> MPAVLGFEGSANKIGVGVVRDGKVLANPRRTYVTPPGTGFLPGDTARHHRAVILDLLQEALTESGLTSQDIDCIAYTKGPGMGAPLVSVAVVARTVAQLWNKPLVGVNHCIGHIEMGRLITGATSPTVLYVSGGNTQVIAYSEHRYRIFGETIDIAVGNCLDRFAR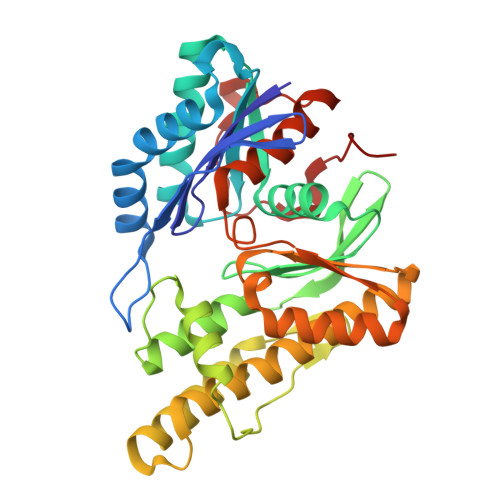VLKISNDPSPGYNIEQMAKRGKKLVELPYTVKGMDVSFSGILSFIEDVAHRMLATGECTPEDLCFSLQETVFAMLVEITERAMAHCGSQEALIVGGVGCNVRLQEMMATMCQERGARLFATDERFCIDNGAMIAQAGWEMFRAGHRTPLSDSGVTQRYRTDEVEVTWRD ethyl 2-[2-octanoyl-3,5-bis(oxidanyl)phenyl]ethanoate | C18 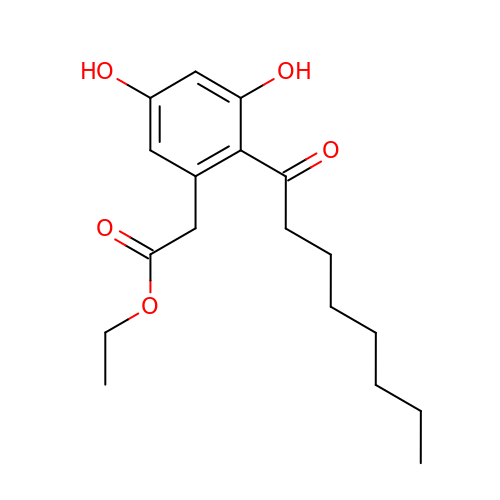H26 O5 | UVVWQQKSNZLUQA-UHFFFAOYSA-N>GPAWPEEKNYHQPAILNSSALRQIAEGTSISEMWQNDLQPLLIERYPGSPGSYAARQHIMQRIQRLQADWVLEIDTFLSQTPYGYRSFSNIISTLNPTAKRHLVLACHYDSKYFSHWNNRVFVGATDSAVPCAMMLELARALDKKLLSLKTVSDSKPDLSLQLIFFDGEEAFLHWSPQDSLYGSRHL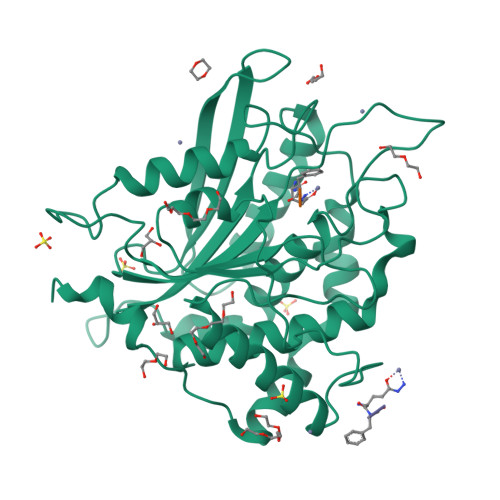AAKMASTPHPPGARGTSQLHGMDLLVLLDLIGAPNPTFPNFFPNSARWFERLQAIEHELHELGLLKDHSLEGRYFQNYSYGGVIQDDHIPFLRRGVPVLHLIPSPFPEVWHTMDDNEENLDESTIDNLNKILQVFVLEYLHL[2x]6-HYDROXYISONICOTINIC ACID 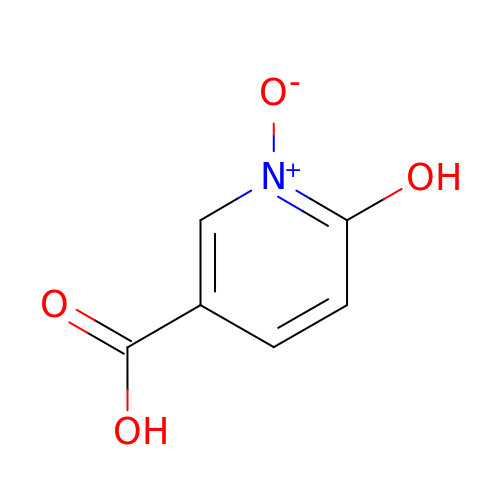N-OXIDE | C6 H5 N O4 | PQTDJLRPWRPPLV-UHFFFAOYSA-N>MSFTPANRAYPYTRLRRNRRDDFSRRLVRENVLTVDDLILPVFVLDGVNQRESIPSMPGVERLSIDQLLIEAEEWVALGIPALALFPVTPVEKKSLDAAEAYNPEGIAQRATRALRERFPELGIITDVALDPFTTHGQCGILDDDGYVLNDVSIDVLVRQALSHAEAGAQVVAPSDMMDGRIGAIREALESAGHTNVRVMAYSAKYASAYYGPFRDAVGSASNLGKGNKATYQMDPANSDEALHEVAADLAEGADMVMVKPGMPYLDIVRRVKDEFRAPTFVYQVSGEYAMHMGAIQNGWLAESVILESLTAFKRAGADGILTYF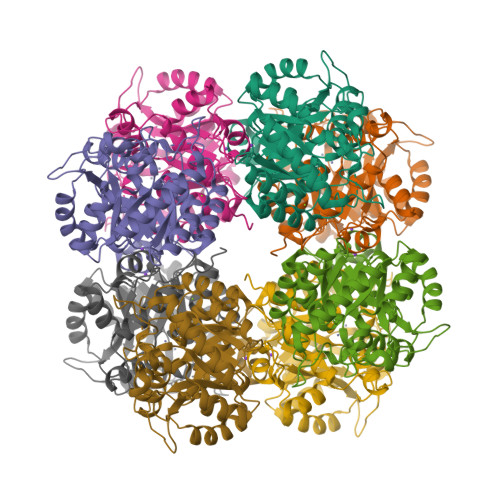AKQAAEQLRRGR[2x]>[4x]GQIQISKHVKDVGLPSIHTPTKTKLQPSVFYDIFPGSKEPAVLTEKDPRLKVDFDSALFSKYKGN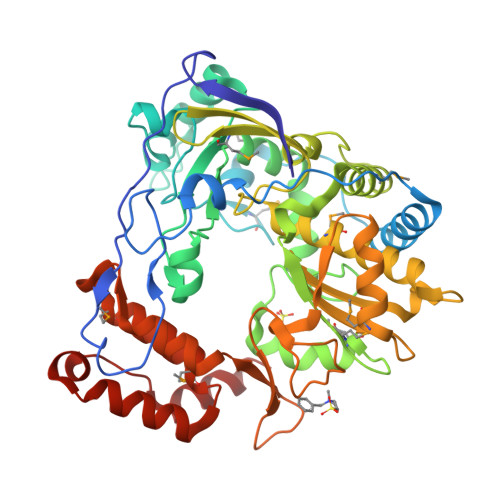TECSLNEHIQVAVAHYSAQLATLDIDPQPIAMEDSVFGMDGLEALDLNTSAGYPYVTLGIKKKDLINNKTKDISKLKLALDKYDVDLPMITFLKDELRKKDKIAAGKTRVIEASSINDTILFRTVYGNLFSKFHLNPGVVTGCAVGCDPETFWSKIPLMLDGDCIMAFDYTNYDGSIHPIWFKALGMVLDNLSFNPTLINRLCNSKHIFKSTYYEVEGGVPSGCSGTSIFNSMINNIIIRTLVLDAYKHIDLDKLKIIAYGDDVIFSYKYKLDMEAIAKEGQKYGLTITPADKSSEFKELDYGNVTFLKRGFRQDDKYKFLIHPTFPVEEIYESIRWTKKPSQMQEHVLSLCHLMWHNGPEIYKDFETKIRSVSAGRALYIPPYELLRHEWYEKF Aurora A kinase (AURKA) is a member of a family of Ser/Thr kinases whose orthologues control progression through mitotic cell division. The localisation of AURKA to microtubules in the mitotic spindle is mediated through its interaction with a protein partner, TPX227. Besides localisation, the AURKA-TPX2 interaction modulates the catalytic activity of AURKA3738. Here, we report the identification of AurkinA, a drug-like inhibitor of AURKA, which binds to a pocket occupied by Y8 and Y10 of TPX2 in the AURKA-TPX2 complex (the Y-pocket).

To provide structural insight into how AurkinA binding might hinder formation of the AURKA-TPX2 complex, we determined the crystal structures of the AURKA catalytic domain in isolation or when liganded to AurkinA. Interestingly, depending on the concentration of reducing agent in buffer, the AURKA kinase domain crystallised either in space group P6122 or in P41212. Analysis of the AURKA structure in hexagonal crystals showed that it remained relatively unchanged when the ATP binding pocket was occupied either with ATP or with JNJ-7706621. The hydrogen bond between Q168 on the αB-helix and the main chain carbonyl of K143 on the G-rich loop, observed consistently in the apo structures, was lost.

> MGRQWALEDFEIGRPLGKGKFGNVYLAREKQSKFILALKVLFKAQLEKAGVEHQLRREVEIQSHLRHPNILRLYGYFHDATRVYLILEYAPLGTVYRELQKLSKFDEQRTATYITELANALSYCHSKRVIHRDIKPENLLLGSAGELKIADFGWSVHAPSSRRTTLCGTLDYLPPEMIEGRMHDEKVDLWSLGVLCYEFLVGKPPFEANTYQETYKRISRVEFTFPDFVTEGARDLISRLLKHNPSQRPMLREVLEHPWITANSSKPHHHHHH> MGSDKIHHHHHHMDRIIEKLDHGWWVVSHEQKLWLPKGELPYGEAANFDLVGQRALQIGEWQGEPVWLVQQQRRHDMGSVRQVIDLDVGLFQLAGRGVQLAEFYRSHKYCGYCGHEMYPSKTEWAMLCSHCRERYYPQIAPCIIVAIRRDDSILLAQHTRHRNGVHTVLAGFVEVGETLEQAVAREVMEESGIKVKNLRYVTSQPWPFPQSLMTAFMAEYDSGDIVIDPKELLEANWYRYDDLPLLPPPGTVARRLIEDTVAM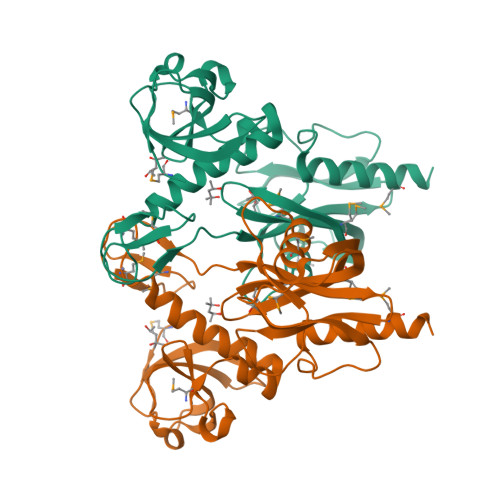CRAEYE2-[[2-[(1~{R},5~{S})-7-phenyl-3,7-diazabicyclo[3.3.1]nonan-3-yl]-1,3-thiazol-4-yl]methyl]-3,4-dihydro-1~{H}-isoquinoline-7-carboxylic 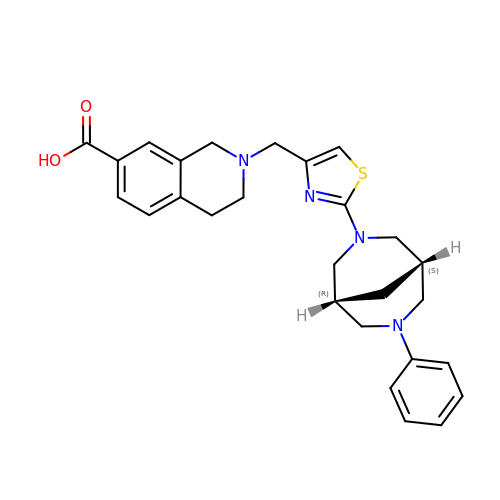acid | C27 H30 N4 O2 S | XGAITRPKSKWJAF-BGYRXZFFSA-N> GSHMTITDVLKNTFNISPKPPRKFIAIDLGTTNSIAYIGGRGIIYNEASVMAYETGTKKLVALGEDARKLIGKTHDKIEIYTPLRNGAITDLRIA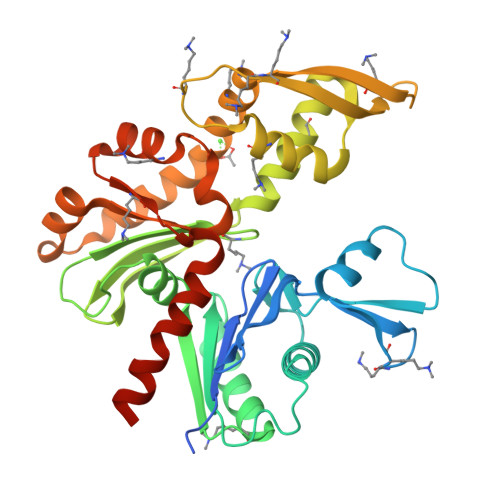EEFIQHIGNRAKVQDVWKGSIVLIACPKSVTELERRAMVEMCKHLGADLVQVEEDTLMAALGAGANIFAPKGTFILDIGGGKTSAGIISAGGIVVSKSIKIAGNYIDEEILKYIRAKHTISIGVVTAEQIKKQIGSLYKGKETKKMVIFGRDVVTGMPKETEILDSEIRKLLISIFSSITQLVTDILESTPAELAGDAVMNGLLVSGGCAQISGLKEFLESYFQIPVKIAKNPQTAVIDGCIAYEKEIRDRLIEENKKNK> GHMPEYDYLFKLLLIGDSGVGKSCLLLRFADDTYTESYISTIGVDFKIRTIELDGKTIKLQIWDTAGQERFRTITSSYYRGAHGIIVVYDVTDQESYANVKQWLQEIDRYASENVNKLLVGNKSDLTTKKVVDNTTAKEFADSLGIPFLETSAKNATNVEQAFMTMAAEIKK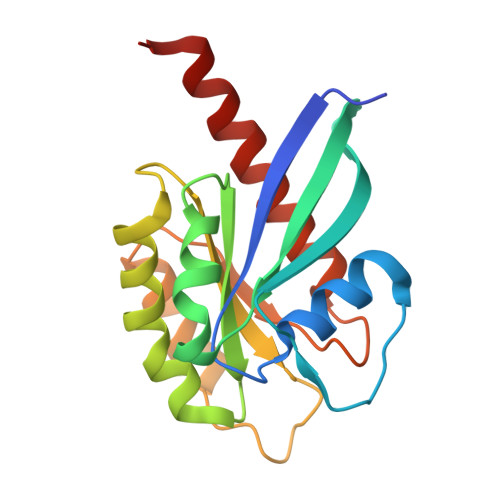RMGLEVLFQ>[2x]METSMVSTTAASSVEHAANTYDFAEAKSGSSIPAKVAAEQANSYSVHGLVTSLAVYQHFSLTVEGGGKTFTGDSGGISIPGVAVLEGTLFTEDLQHLYSDTV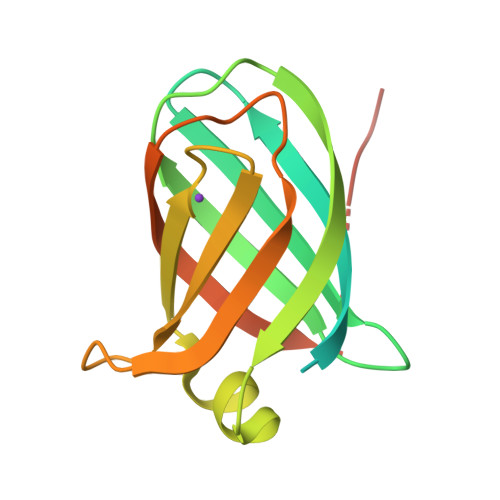SFEYNAVGPYLNINFFDSHGTLLGHVQSGSIGTVSGIGGGTGGWQPNSSSVDKLAAALEHHHHHH>GPGSRDVEMEEMIEQLQEKVHELERQNEVLKN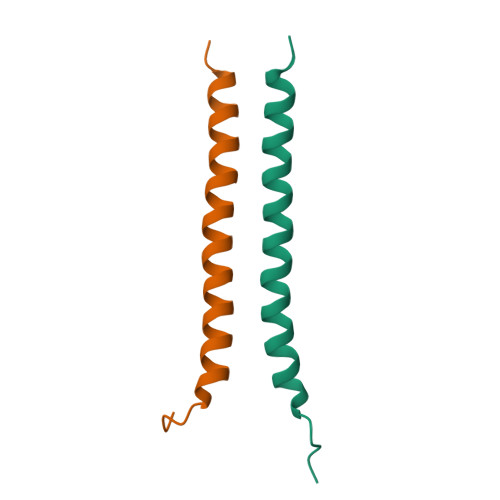RLISAKQQLQVQG[2x]>[2x]MSEFNITETYLRFLEEDTEMTMPIAAIEALVTLLRIKTPETAAEMINTIKSSTEELIKSIPNSVSLRAGCDIFMRFVLRNLHLYGDWENCKQHLIENGQLFVSRAKKSRNKIAEIGVDFIADDDIILVHGYSRAVFSLLNHAANKFIRFRCVVTESRPSKQGNQLYTLLEQKGIPVTLIVDSAVGAVIDKVDKVFVGAEGVAESGGIINLVGTYSVGVLAHNARKPFYVVTESHKFVRMFPLSSDDLPMAGPPLDFTRRTDDLEDALRGPTIDYTAQEYITALITDLGVLTPSAVSEELIKMWYD;>[2x]MSESEAKSRSATPPSKAKQATPTTTAAANGEKKLTNKELKELKKQEKAAKRAAMKQANGISIEQQQQQAQMKKEKKQLQREQQQKREQKQKNANKKKQNERNVKKSTLFGHLETTEERRATILALTSAVSSPKTSRITAAGLMVPVVASALSGSNVLTASSLMPVGPNASSTVSASAPASTTTTLPASSAALSAGTSSASTNTPTAIQQEIASSNASDVAKTLASISLEAGEFNVIPGISSVIPTVLEQSFDNSSLISSVKELLLNKDLIHPSILLLTSHLAHYKIVGSIPRCIAMLEVFQIVIKDYQTPKGTTLSRNLTSYLSHQIDLLKKARPLSVTMGNAIRWLKQEISLIDPSTPDKAAKKDLCEKIGQFAKEKIELADQLIIDNASTQIEESTTIVTYGSSKVLTELLLHNAISLKKNIKVIVVDSRPLFEGRKMAETLRNAGVNVMYALITSLDTIFNMDVDYVFLGAHSILSNGFLYSRAGTAMLAMSAKRRNIPVLVCCESLKFSQRVQLDSVTFNELADPNDLVNIDYENPVERRGNKGALLNQFIKERKFEKKKLAMENKPKGNKIGGKKGSEGESKDASNEEDSNSKNILDGWQELPSLNIVNILYDLTPPEYIKKVITEFGALPPSSVPVILREYKGSA;>MSSQAFTSVHPNAATSDVNVTIDTFVAKLKRRQVQGSYAIALETLQLLMRFISAARWNHVNDLIEQIRDLGNSLEKAHPTAFSCGNVIRRILAVLRDEVEEDTMSTTVTSTSVAEPLISSMFNLLQKPEQPHQNRKNSSGSSSMKTKTDYRQVAIQGIKDLIDEIKNIDEGIQQIAIDLIHDHEILLTPTPDSKTVLKFLITARERSNRTFTVLVTEGFPNNTKNAHEFAKKLAQHNIETLVVPDSAVFALMSRVGKVIIGTKAVFVNGGTISSNSGVSSVCECAREFRTPVFAVAGLYKLSPLYPFDVEKFVEFGGSQRILPRMDPRKRLDTVNQITDYVPPENIDIYITNVGGFNPSFIYRIAWDNYKQIDVHLDKNKA[2x];>MAGKKGQKKSGLGNHGKNSDMDVEDRLQAVVLTDSYETRFMPLTAVKPRCLLPLANVPLIEYTLEFLAKAGVHEVFLICSSHANQINDYIENSKWNLPWSPFKITTIMSPEARCTGDVMRDLDNRGIITGDFILVSGDVLTNIDFSKMLEFHKKMHLQDKDHISTMCLSKASTYPKTRTIEPAAFVLDKSTSRCIYYQDLPLPSSREKTSIQIDPELLDNVDEFVIRNDLIDCRIDICTSHVPLIFQENFDYQSLRTDFVKGVISSDILGKHIYAYLTD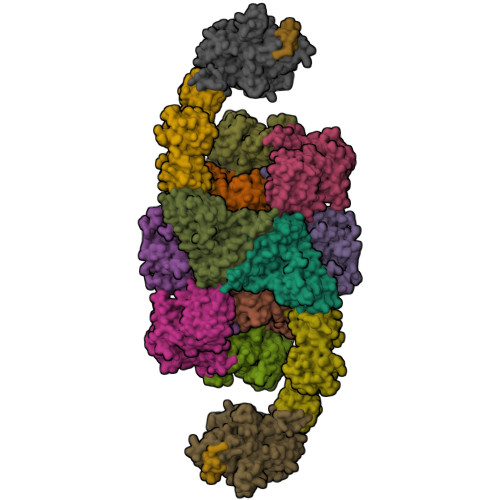EYAVRVESWQTYDTISQDFLGRWCYPLVLDSNIQDDQTYSYESRHIYKEKDVVLAQSCKIGKCTAIGSGTKIGEGTKIENSVIGRNCQIGENIRIKNSFIWDDCIIGNNSIIDHSLIASNATLGSNVRLNDGCIIGFNVKIDDNMDLDRNTKISASPLKNAGSRMYDNESNEQFDQDLDDQTLAVSIVGDKGVGYIYESEVSDDEDSSTEACKEINTLSNQLDELYLSDDSISSATKKTKKRRTMSVNSIYTDREEIDSEFEDEDFEKEGIATVERAMENNHDLDTALLELNTLRMSMNVTYHEVRIATITALLRRVYHFIATQTLGPKDAVVKVFNQWGLLFKRQAFDEEEYIDLMNIIMEKIVEQSFDKPDLILFSALVSLYDNDIIEEDVIYKWWDNVSTDPRYDEVKKLTVKWVEWLQNADEESSSEEE[2x];>[2x]MSIQAFVFCGKGSNLAPFTQPDFPFQTQNKDSTAATSGDKLNELVNSALDSTVINEFMQHSTRLPKALLPIGNRPMIEYVLDWCDQADFKEISVVAPVDEIELIESGLTSFLSLRKQQFELIYKALSNSNHSHHLQDPKKINFIPSKANSTGESLQKELLPRINGDFVILPCDFVTDIPPQVLVDQFRNRDDNNLAMTIYYKNSLDSSIDKKQQQKQKQQQFFTVYSENEDSERQPILLDVYSQRDVTKTKYLQIRSHLLWNYPNLTVSTKLLNSFIYFCSFELCQLLKLGPQSMSRQASFKDPFTGNQQQQNPPTTDDDEDRNHDDDDDYKPSATSIQPTYFKKKNDLILDPINCNKSLSKVFRDLSRRSWQHSKPREPIGIFILPNETLFIRANNLNAYMDANRFVLKIKSQTMFTKNIQIQSAAIGADAIVDPKCQISAHSNVKMSVLGTQANIGSRCRVAGSLLFPGVHLGDEVILENCIIGPMAKIGSKCKLSNCYIEGHYVVEPKNNFKGETLANVYLDEDEEDELIYDDSVIAGESEIAEETDSDDRSDEDSDDSEYTDEYEYEDDGLFER;>[2x]MSTSHCRFYENKYPEIDDIVMVNVQQIAEMGAYVKLLEYDNIEGMILLSELSRRRIRSIQKLIRVGKNDVAVVLRVDKEKGYIDLSKRRVSSEDIIKCEEKYQKSKTVHSILRYCAEKFQIPLEELYKTIAWPLSRKFGHAYEAFKLSIIDETVWEGIEPPSKDVLDELKNYISKRLTPQAVKIRADVEVSCFSYEGIDAIKDALKSAEDMSTEQMQVKVKLVAAPLYVLTTQALDKQKGIEQLESAIEKITEVITKYGGVCNITMPPKAVTATEDAELQALLESKELDNRSDSEDDEDESDDE;>MSSDLAAELGFDPALKKKKKTKKVIPDDFDAAVNGKENGSGDDLFAGLKKKKKKSKSVSADAEAEKEPTDDIAEALGELSLKKKKKKTKDSSVDAFEKELAKAGLDNVDAESKEGTPSANSSIQQEVGLPYSELLSRFFNILRTNNPELAGDRSGPKFRIPPPVCLRDGKKTIFSNIQDIAEKLHRSPEHLIQYLFAELGTSGSVDGQKRLVIKGKFQSKQMENVLRRYILEYVTCKTCKSINTELKREQSNRLFFMVCKSCGSTRSVSSIKTGFQATVGKRRRM[2x];>[2x]MSDLQDQEPSIIINGNLEPVGEPDIVEETEVVAQETQETQDADKPKKKVAFTGLEEDGETEEEKRKREFEEGGGLPEQPLNPDFSKLNPLSAEIINRQATINIGTIGHVAHGKSTVVRAISGVQTVRFKDELERNITIKLGYANAKIYKCQEPTCPEPDCYRSFKSDKEISPKCQRPGCPGRYKLVRHVSFVDCPGHDILMSTMLSGAAVMDAALLLIAGNESCPQPQTSEHLAAIEIMKLKHVIILQNKVDLMREESALEHQKSILKFIRGTIADGAPIVPISAQLKYNIDAVNEFIVKTIPVPPRDFMISPRLIVIRSFDVNKPGAEIEDLKGGVAGGSILNGVFKLGDEIEIRPGIVTKDDKGKIQCKPIFSNIVSLFAEQNDLKFAVPGGLIGVGTKVDPTLCRADRLVGQVVGAKGHLPNIYTDIEINYFLLRRLLGVKTDGQKQAKVRKLEPNEVLMVNIGSTATGARVVAVKADMARLQLTSPACTEINEKIALSRRIEKHWRLIGWATIKKGTTLEPIA> TTTVTSEDHFMTFYNENNKKL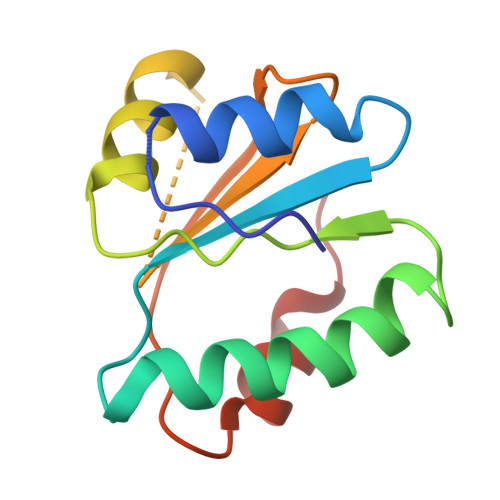IVVDVYPGWSGPCTAMYPTYNQLMISIDDFEKRIDILLLDQDKLVTYKNDKFHATCQPKFLFISEGKIIDEVLGTNIPVFIEKVNKYIPLS Bromodomains (BRDs) are protein interaction modules that specifically recognize ε-N-lysine acetylation motifs, a key event in the reading process of epigenetic marks. The 61 BRDs in the human genome cluster into eight families based on structure/sequence similarity. Despite large sequence variations, all BRD modules share a conserved fold that comprises a left-handed bundle of four α helices (αZ, αA, αB, αC), linked by loop regions of variable length (ZA and BC loops), which line the Kac binding site and determine binding specificity. The four helices form a deep cavity that is extended by the two loop regions (ZA and BC loops), creating a largely hydrophobic Kac binding pocket.

BRDs are evolutionarily conserved and present in diverse nuclear proteins comprising HATs (GCN5, PCAF), ATP-dependent chromatin-remodeling complexes (BAZ1B), helicases (SMARCA), methyltransferases (MLL, ASH1L), transcriptional coactivators (TRIM/TIF1, TAFs) transcriptional mediators (TAF1), nuclear-scaffolding proteins (PB1), and the BET family (Muller et al., 2011). The most notable structural difference within the BRD core fold is a hairpin insertion located between helix αZ and the ZA loop that is present in all family VIII members. The proximity to the Kac binding site suggests that this insert may play a role in recruitment of acetylated binding partners. The nuclear body protein SP140 as well as the related protein LOC93349 and PCAF showed nonspecific binding to most peptides. In contrast, the second, fourth, fifth, and sixth BRD of PB1, MLL, and TRIM28 interacted with only a few histone Kac peptides.

>SMSGISPKKSKYMTPMQQKLNEVYEAVKNYTDKRGRRLSAIFLRLPSRSELPDYYLTIKKPMDMEKIRSHMMANKYQDIDSMVEDFVMMFNNACTYNEPESLIYKDALVLHKVLLETRRDLEGD[2x]>QEPQPEQDPFELSGKWITSYIGSSDLEKIGENAPFQVFMRSIEFDDKESKVYLNFFSKENGICEEFSLIGTKQEGNTYDVNYAGNNKFVVSYASETALIISNINVDEEGDKTIMTGLLGKGTDIEDQDLEKFKEVTRENGI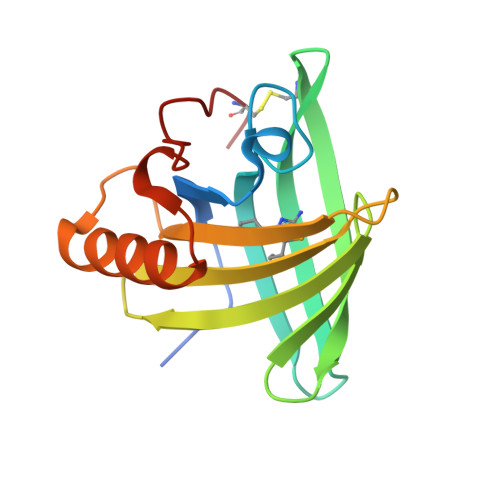PEENIVNIIERDDCPA[2x]>[2x]HHNKEWLSKPTDKRRLSELTQIWWDLKGKHEEHGKSNLGKIEIFTKITN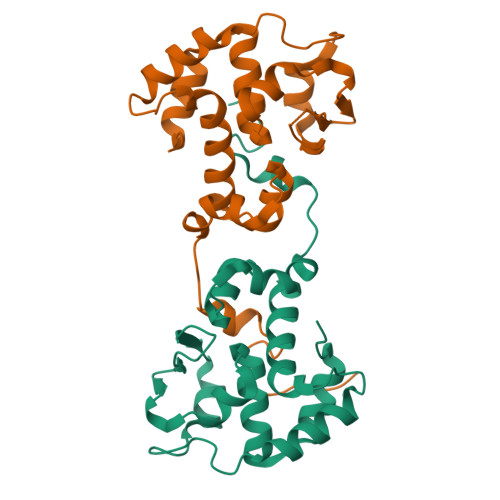DPCAFQITKSLISQYCATRRSQGIKPSSINRDLTCISGMFTALIEAELFFGEHPIRGTKRLKEEKPETGYLTQEEIALLLAALDGDNKKIAILCLSTGARWGEAARLKAENIIHNRVTFVKTKTNKPRTVPISEAVAKMIADNKRGFLFPDADYPRFRRTMKAIKPDLPMGQATHALRHSFATHFMINGGSIITLQRILGHTRIEQTMVYAHFAPEYLQDAISLNPLRGGTEAESVHTVSTVE> GIGTGFPFDPHYVEVLGERMHYVDVGPRDGTPVLFLHGNPTSSYVWRNIIPHVAPTHRCIAPDLIGMGKSDKPDLGYFFDDHVRFMDAFIEALGLEEVVLVIHDWGSALGFHWAKRNPERVKGIAFMEFIRPIPTWDEWPEFARETFQAFRTTDVGRKLIIDQNVFIEGTLPMGVVRPLTEVEMDHYREPFLNPVDREPLWRFPNELPIAGEPANIVALVEEYMDWLHQSPVPKLLFWGTPGVLIPPAEAARLAKSLPNCKAVDIGPGLNLLQEDNPDLIGSEIARWLSTLEI

The self-labeling protein tags (SLPs) HaloTag7, SNAP-tag, and CLIP-tag allow the covalent labeling of fusion proteins with synthetic molecules for applications in bioimaging and biotechnology. The three most popular SLPs are HaloTag7 (HT7),14 SNAP-tag (SNAP),15 and CLIP-tag (CLIP)16. To guide the selection of an SLP–substrate pair and provide guidelines for the design of substrates, we report a systematic and comparative study of the labeling kinetics and substrate specificities of HaloTag7, SNAP-tag, and CLIP-tag. We complement these kinetic studies by reporting crystal structures of HT7 and SNAP covalently labeled with rhodamine-based fluorophores, providing a detailed understanding of their substrate preferences.

HT7 was engineered from a bacterial dehalogenase (DhaA from Rhodococcus sp.), an enzyme that can hydrolyze halogenated alkanes. Inactivating the second catalytic step of its enzymatic reaction (mutation H272N in HT7) abolished the hydrolysis of the ester formed with an active site aspartate residue and created an SLP. HT7 reacts specifically with chloroalkane-PEG (CA) molecules resulting in covalent bonding of the alkane chain to the reactive aspartate and release of a chloride ion. In addition to the conventional α/β-hydrolase topology, HT7 features an extra capping domain made of six α-helices (Hlx4–9) that partially cover the catalytic site and form an entry channel for the CA substrate. After reaction, the PEG-alkane ligand is buried in the protein, while the xanthene moiety of the dye lays on the distorted α-helix 8 (Hlx8) in a conformation partially constrained by the crystal packing. The alkane-fluorophore is positioned by the Hlx6–turn–Hlx7–turn–Hlx8 motif of the HT7 capping domain from which T172Hlx8 and, to a lesser extent, T148Hlx6 form hydrogen bonds with the oxygen and the nitrogen of the amide bond linking PEG-alkane and fluorophore. CA-TMR and CA-CPY have similar conformations in both structures with only minor differences in their torsion angles. The direct comparison of SNAP and HT7 reveals that HT7 features significantly higher labeling rate constants with various fluorescent rhodamine derivatives. These differences in reactivity can be explained by specific interactions of the rhodamine’s xanthene ring with selected surface residues of HT7. The mechanism underlying the equilibrium shift from the spirocyclic nonfluorescent to the zwitterionic fluorescent form is not yet fully understood, but our results indicate that the planar, zwitterionic form of rhodamines (e.g., TMR and CPY) features energetically favorable interactions with the HT7 surface, thus potentially favoring this state of the fluorophore when attached to the protein.> MGSMIKTIAFGRYELDTWYHSPYPEEYARLGRLYMCEFCLKYMKSQTILRRHMAKCVWKHPPGDEIYRKGSISVFEVDGKKNKIYCQNLCLLAKLFLDHKTLYYDVEPFLFYVMTEADNTGCHLIGYFSKEKNSFLNYNVSCILTMPQYMRQGYGKMLIDFSYLLSKVEEKVGSPERPLSDLGLISYRSYWKEVLLRYLHNFQGKEISIKEISQETAVNPVDIVSTLQALQMLKYWKGKHLVLKRQDLIDEWIAKEAKRSNSNKTMDPSCLKWTPPKAS;> GSLTYAQAQGMVE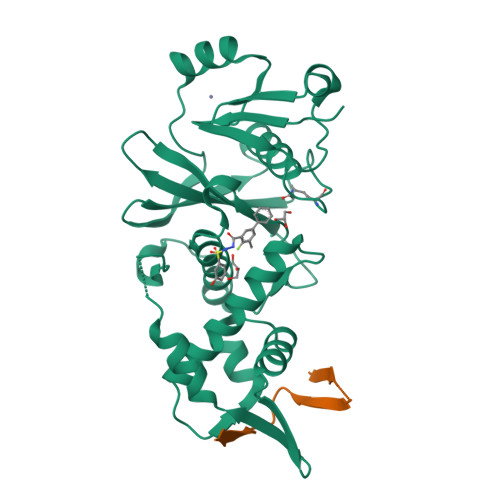IEIEGRLHRISIFDPLEIILEDDLTAQEMSECNSNKENS> GSAFPMTMDEKYVNSIWDLLKNAIQEIQRKNNSGLSFEELYRNAYTMVLHKHGEKLYTGLREVVTEHLINKVREDVLNSLNNNFLQTLNQAWNDHQTAMVMIRDILMYMDRVYVQQNNVENVYNLGLIIFRDQVVRYGCIRDHLRQTLLDMIARERKGEVVDRGA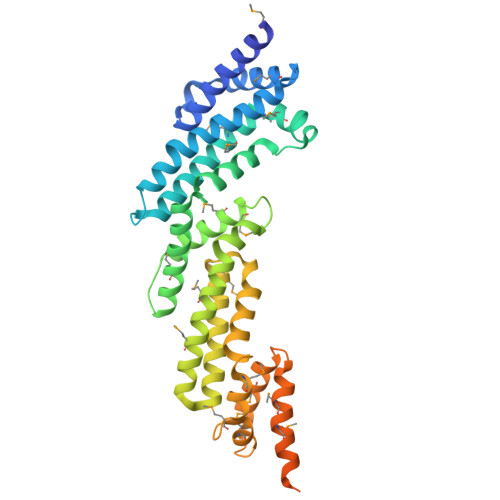IRNACQMLMILGLEGRSVYEEDFEAPFLEMSAEFFQMESQKFLAENSASVYIKKVEARINEEIERVMHCLDKSTEEPIVKVVERELISKHMKTIVEMENSGLVHMLKNGKTEDLGCMYKLFSRVPNGLKTMCECMSSYLREQGKALVSEEGEGKNPVDYRQGLDDLKSRFDRFLLESFNNDRLFKQTIAGDFEYFLNLN A hallmark of all motile M. xanthus cells is the accumulation of MglA-GTP at the leading pole where it activates motility, while MglA-GDP is found diffusely in the cytosol. This localization pattern arises due to the GAP activity of MglB, which is located at the lagging pole where it inactivates MglA-GTP and depletes it from this pole. The ability of MglA to hydrolyze GTP is essential for motility regulation. To gain insight into the structural landscape of M. xanthus MglA, we determined the crystal structures of MglA in different nucleotide states, which uncovered that MglA can adopt three conformations: inactive MglA-GDP, active MglA-GTPγS, whose structure had not been determined before, and an unusual conformation combining inactive and active features.

Remarkably, we trapped MglA in a mixed state in which switch 1 is in the inactive conformation and switch 2 is in the active conformation, an inactive/active combination never observed in a small GTPase before. The nucleotide-binding site contains GDP and a ligand tentatively ascribed to inorganic phosphate (Pi) with two partially occupied positions, possibly arising from spontaneous hydrolysis of GTPγS over time. There is no Mg2+ in this structure, as its binding site is occluded by the retracted switch 1. Structures of small GTPases with bound GDP-Pi have shown that this state retains the conformation of the GTP-bound precursors. Accordingly, overlay with MglA-GTPγS shows that GTP can readily be accommodated in the mixed MglA conformation, suggesting that MglA can adopt two distinct GTP-bound states. The observation that the mixed MglA conformation observed in the crystal contains GDP and Pi raises the possibility that the MglB-refractory MglA species is a post-hydrolysis intermediate resulting from spontaneous hydrolysis of GTP into GDP-Pi. However, analysis of the nucleotide content of MglB-resistant MglA samples showed that the major bound nucleotide was GTP. Several lines of evidence suggest that the MglA-GTP* species identified biochemically and in vivo corresponds to the mixed inactive/active conformation seen in the crystal: (1) considering that all known crystal structures of small GTPases bound to GDP-Pi retain the conformation of their GTP-bound precursor, and that the mixed structure, although it contains GDP-Pi, can readily accommodate GTP, it is likely that the mixed structure derives from a GTP-bound MglA species with the same mixed conformation. (2) The retracted conformation of switch 1 in the mixed form does not allow it to establish the interactions seen in the MglA/MglB complex, which can readily explain its resistance to MglB-stimulated GTP hydrolysis. Further work is needed to prove that the feedback loop operates in vivo, but the observation that an MglA-YFP population remains immobilized at the cell pole when the diffusible MglB3M mutant is expressed strongly suggests that the MglA-GDP/MglA-GTP*/MglA-GTP cycle is required for functional MglA oscillations.

>MSFINYSSREINCKIVYYGPGLCGKTTNLQYIYNKTAAETKGKLISLSTETDRTLFFDFLPLSLGEIRGFKTRFHLYTVPGQVFYDASRKLILKGVDGVVFVADSQIERMEANMESLENLRINLAEQGYDLNKIPYVIQYNKRDLPNAVTVEEMRKALNHRNIPEYQAVAPTGVGVFDTLKAVAKLVLTELKKGGHHHHHH[2x]> MSKFGRKVPSNAKSQHNFSVIPSANIQRSVFNRSSGYKTTFDAGYLIPVFLDEALPGDTFHLKTSVLARLSTPVVPFMDNLRLDIQYFSVPYRLVWDNWQKFNGEQKNPGDSTDYLIPQIKAPAGGFPVGSLADYFGVPTGVENISVSALPFRAYNLIYNEWYRDENLINSAPLPLGDEEETGLANFPLRKRAKRHDYFTSALPWPQKGEGVEIGLGVPPSYTLEYPYYKEGMGFISSNYGASGNIGRTFPTYIARSSVGDDSSSNIGNAAYFSEGLENGINFPNAPARGRYDVLGGFDPNTPPVTLKKEGGEVVDNLTINSLRQAFQLQRLLERDARGGTRYIEIIRSHFGVISPDARVQRPEYLGSGSFDININPVLQNSATTDASPQGNLAAYGVSGGVNRGFSHSFVEHCFVIGLVSVRADLTYQQGIPRMFSRQTRFDFYWPALAHLGEQAILNKEIYAQGNAKDDEVFGYQERYAEYRYRPSQITGKLRSTDPQSLDVWHLAQRFDSLPALNQEFIEENPPM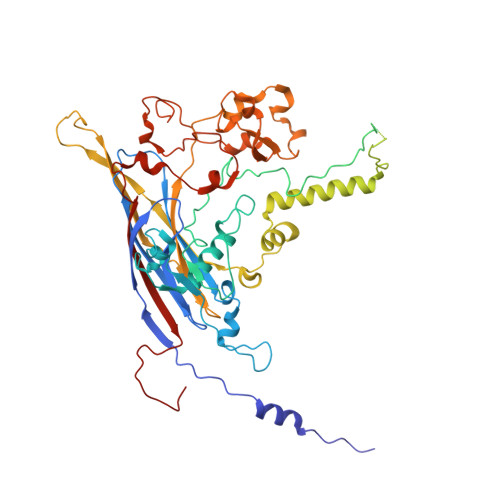KRVLAVQDEPQFIMDAFFDLKCVRPMPVYSVPGLIDHF>[8x]GSMEGPAGYLRRADVAQLTQELGTAFFQQQQLPAAMADTFLEHLCLLDIDSEPVAARSTSIIATIGPASRSVERLKEMIKAGMNIARLNFSHGSHEYHAESIANVRE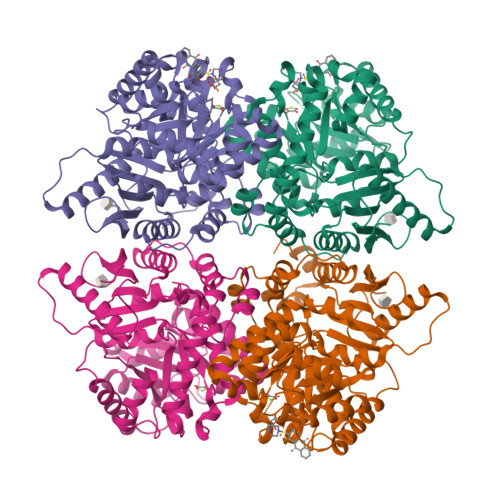AVESFAGSPLSYRPVAIALDTKGPGSGPGLSEQDVRDLRFGVEHGVDIVFASFVRKASDVAAVRAALGPEGHGIKIISKIENHEGVKRFDEILEVSDGIMVARGDLGIEIPAEKVFLAQKMMIGRCNLAGKPVVCATQMLESMITKPRPTRAETSDVANAVLDGADCIMLSGETAKGNFPVEAVKMQHAIAREAEAAVYHRQLFEELRRAAPLSRDPTEVTAIGAVEAAFKCCAAAIIVLTTTGRSAQLLSRYRPRAAVIAVTRSAQAARQVHLCRGVFPLLYREPPEAIWADDVDRRVQFGIESGKLRGFLRVGDLVIVVTGWRPGSGYTNIMRVLSIS>MSETWLPTLVTATPQEGFD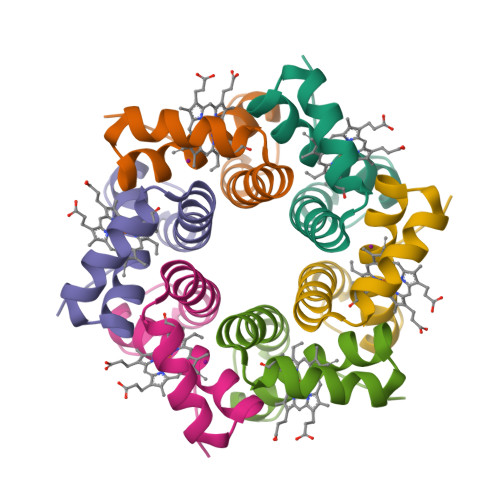LAVKLSRIAVKKTQPDAQVRDTLRAVYEKDANALIAVSAVVATHFQTIAAANDYWKD[8x]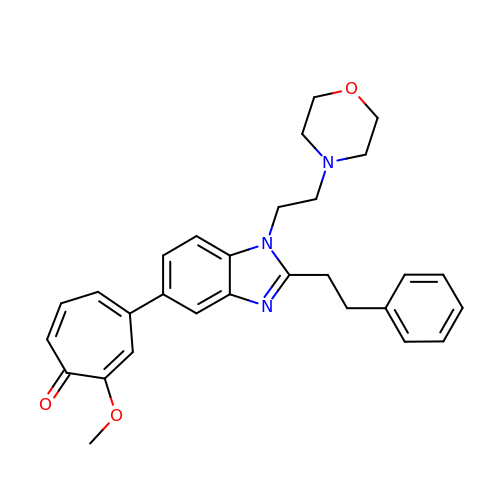2-methoxy-4-{1-[2-(morpholin-4-yl)ethyl]-2-(2-phenylethyl)-1H-benzimidazol-5-yl}cyclohepta-2,4,6-trien-1-one | C29 H31 N3 O3 | ZSTNBLSPAMZIQD-UHFFFAOYSA-N>[4x]NTKYNKEFLLYLAGFVDGDGSIIAQIKPNQSYKFKHQLSLTFQVTQKTQ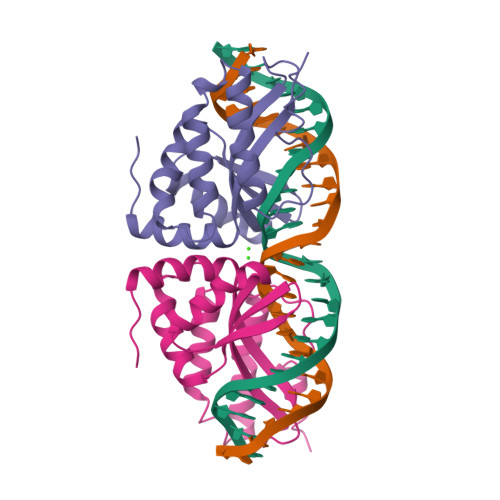RRWFLDKLVDEIGVGYVRDRGSVSDYILSEIKPLHNFLTQLQPFLKLKQKQANLVLKIIEQLPSAKESPDKFLEVCTWVDQIAALNDSKTRKTTSETVRAVLD>[4x]SNAMSSSSSPPHQLNHFSDVANKAANAAGDVIRKYFRKNNFDIIHKNDLSPVTIADQSAEEAMVSVILDNFPSHAVYGEEKGWRCKQDSADYVWVLDPIDGTKSFITGKPLFGTLIALLQNGTPILGIIDQPVLKERWIGITGKRTTLNGQEVSTRTCADLSQAYLYTTSPHLFSGDAEEAFIR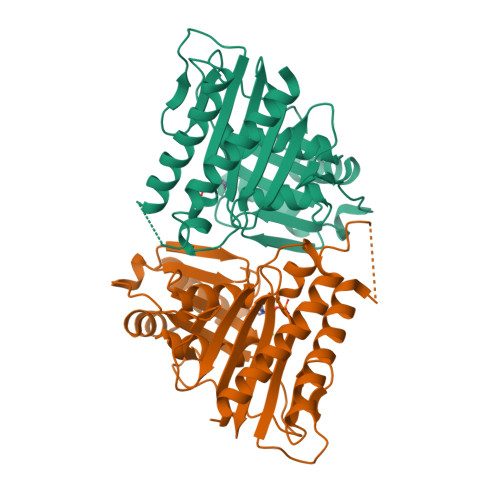VRDKVKIPLYGCDCYAYALLSSGFVDLVVESGLKPYDFLALIPVIEGSGGVITDWKGHQLRWEASPLSIATSFNVVAAGDKQIHQQALDSLQW> MSSHTPKLDSCGAEPIHIPGAIQEHGALLVLSAREFSVVQASDNLANYIGVDLPIGAVATEANLPFISVLSAWYSGEESNFRYAWAEKKLDVSAHRSGTLVILEVEKAGVGESAEKLMGELTSLAKYLNSAPSLEDALFRTAQLVSSISGHDRTLIYDFGLDWSGHVVAEAGSGALPSYLGLRFPAGDIPPQARQLYTINRLRMIPDVDYKPVPIRPEVNAETGAVLDMSFSQLRSVSPVHLEYMRNMGTAASMSVSIVVNGALWGLIACHHATPHSVSLAVREACDFAAQLLSMRIAMEQSSQDASRRVELGHIQARLLKGMAAAEKWVDGLLGGEGEREDLLKQVGADGAALVLGDDYELVGNTPSREQVEELILWLGEREIADVFATDNLAGNYPTAAAYASVASGIIAMRVSELHGSWLIWFRPEVIKTVRWGGDPHK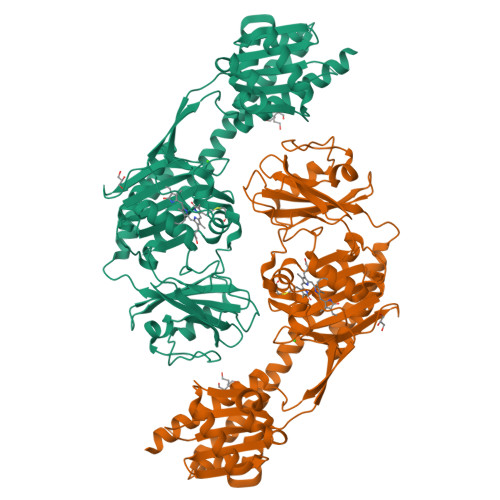TVQESGRIHPRKSFEIWKEQLRNTSFPWSEPELAAARELRGAIIGIVLRKTEEHHHHHH>[16x]GSDEDTYYLQV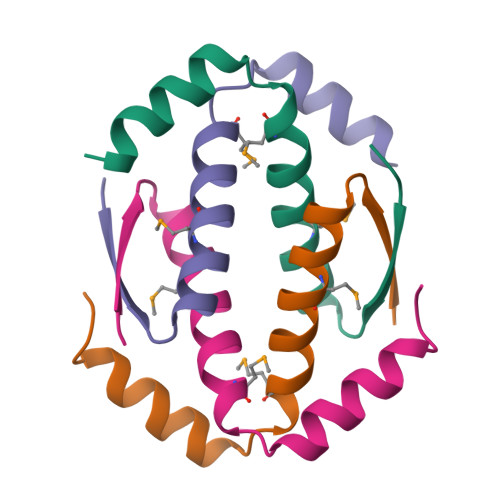RGRENFEILMKLKESLELMELVPQPLVDSYRQQQQLLQRP>[2x]ASPRANDAPIVLLHGFTGWGREEMLGFKYWGGVRGDIEQWLNDNGYRTYTLAVGPLSSNWDRACEAYAQLVGGTVDYGAAHAAKHGHARFGRTYPGLLPELKRGGRVHIIAHSQGGQTARMLVSLLENGSQEEREYAKEHNVSLSPLFEGGHRFVLSVTTIATPHDGTTLVNMVDFTDRFFDLQ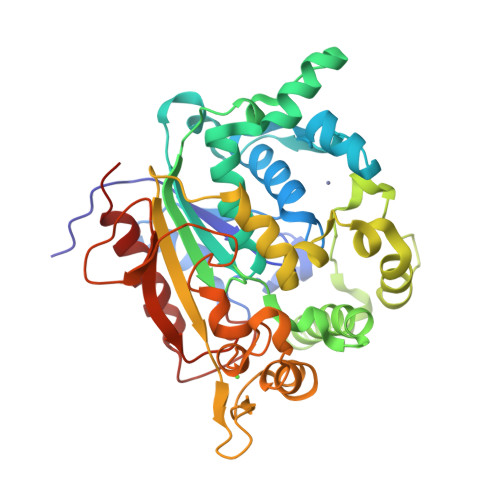KAVLEAAAVASNAPYTSEIYDFKLDQWGLRREPGESFDHYFERLKRSPVWTSTDTARYDLSVPGAETLNRWVKASPNTYYLSFSTERTYRGALTGNYYPELGMNAFSAIVCAPFLGSYRNAALGIDSHWLGNDGIVNTISMNGPKRGSNDRIVPYDGTLKKGVWNDMGTYNVDHLEVIGVDPNPSFNIRAFYLRLAEQLASLRP> GPLGSEEDVPENNGILISIKEVINAEFSRDGTIHSSELKGVLELRINDHDLSHSNLKLADSIDVRDKSFQFKTHPNIDKQSFLSTKLISLRDKSKAFP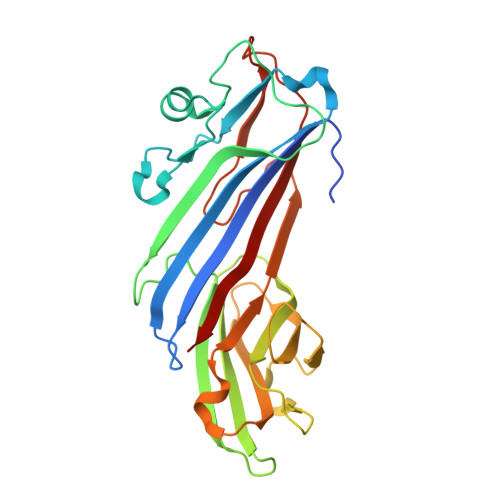ANDQSLGVLRWRKVAPAEDDSLIPLTLTTAVSPSESQQGFDVIIEYESVLETELADVIFTIPVFPQEPVDINTESSTCSDAEVVNMDQEMGTSIKISKIAANDAGALAFTIEAPYEDALYPMTVSFQESTRDKLAKSFTGMAIQSVVMANDHDQELPYDVITSLKSDEYLVQ> SVSIGYLLVKHSQTDQEPMCPVGMNKLWSGYSLLYFEGQEKAHNQDLGLAGSCLARFSTMPFLYCNPGDVCYYASRNDKSYWLSTTAPLPMMPVAEDEIKPYISRCSVCEAPAIAIAVHSQDVSIPHCPAGWRSLWIGYSF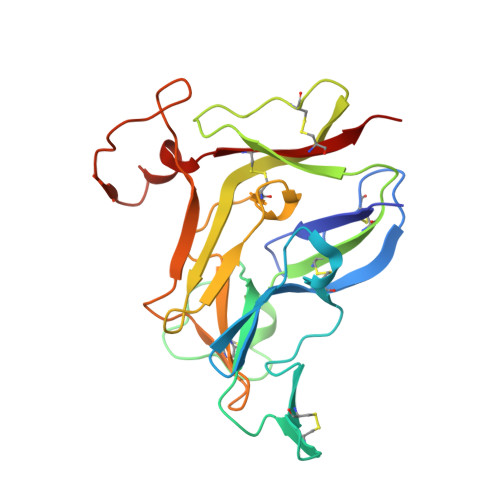LMHTAAGDEGGGQSLVSPGSCLEDFRATPFIECNGGRGTCHYYANKYSFWLTTIPEQSFQGSPSADTLKAGLIRTHISRCQVCMKNL>MARCTGSVELGGLFKSGTGCDHMLSKDIIKLLNEQVNKEMNSSNLYMSMSSWCYTHSLDGAGLFLFDHAAEEYEHAKKLIVFLNENNVPVQLTSISAPEHKFEGLTQIFQKAYEHEQHISESINNIVDHAIKSKDHATFNFLQWYVSEQH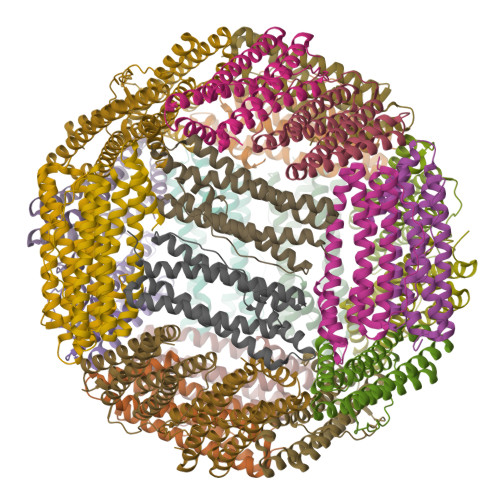EEEVLFKDILDKIELIGNENHGLYLADQYVKGIAKSRKS[8x]> SLGIFPTVEKLVEEMREQL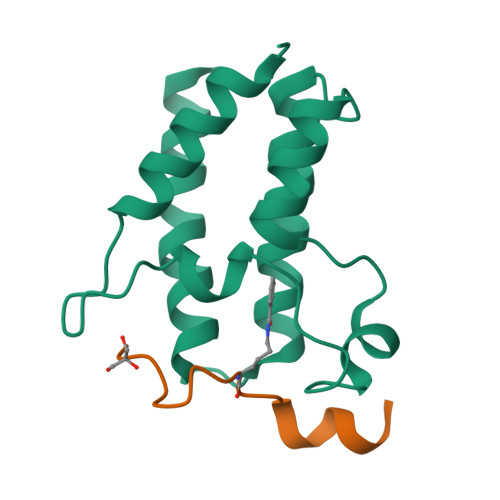DEVDSHPRTSIFEKLPSKRDYPDYFKVIEKPMAIDIILKNCKNGTYKTLEEVRQALQTMFENARFYNEEGSWVYVDADKLNEFTDEWFKEHSS;> TARKSTGGKAPRKQLASY>MAHHHHHHMTAEVLFARWRDRIESQLDAALPSPAEAPQRLHQAMRYSVLGGG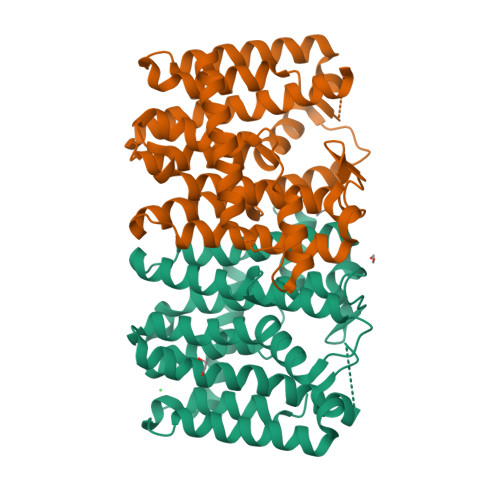KRMRPLLVYASGHLFGTQPESLDAAAMSVELIHAYSLVHDDLPAMDDDALRRGKPTTHVAFDEATAILAGDALQTRAFGLLADAPLPATLRVACLQTLAHASGASGMCGGQALDIDATGQQQTLAALTRMHALKTGALIRAAVRMGALCGQAHEPQLAQLDSFADALGLAFQVRDDILDVEASSEQLGKTAGKDQAQDKSTFPALLGMDGAKAQLHELAARMQSILARYGEEADALRALATLAVERDH[2x]>MGASARLLRAVIMGAPGSGKGTVSSRITTHFELKHLSSGDLLRDNMLRGTEIGVLAKAFIDQGKLIPDDVMTRLALHELKNLTQYSWLLDGFPRTLPQAEALDRAYQIDTVINLNVPFEVIKQRLTARWIHPASGRVYNIEFNPPKTVGIDDLTGEPLIQREDDKPETVIKRLKAYEDQTKPVL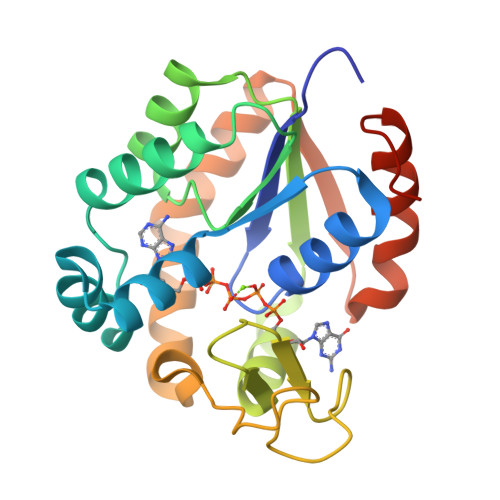EYYQKKGVLETFSGTETNKIWPYVYAFLQTKVPQRSQKASVTP[6x]> FNLDTEELTAFRVDSAGFGDSVVQYANSWVVVGAPQKITAANQTGGLYQCGYSTGACEPIGLQVPPEAVNMSLGLSLASTTSPSQLLACGPTVHHECGRNMYLTGLCFLLGPTQLTQRLPVSRQECPRQEQDIVFLIDGSGSISSRNFATMMNFVRAVISQFQRPSTQFSLMQFSNKFQTHFTFEEFRRSSNPLSLLASVHQLQGFTYTATAIQNVVH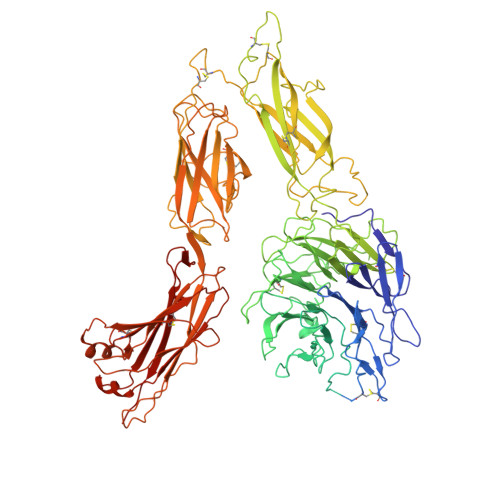RLFHASYGARRDAAKILIVITDGKKEGDSLDYKDVIPMADAAGIIRYAIGVGLAFQNRNSWKELNDIASKPSQEHIFKVEDFDALKDIQNQLKEKIFAIEGTETTSSSSFELEMAQEGFSAVFTPDGPVLGAVGSFTWSGGAFLYPPNMSPTFINMSQENVDMRDSYLGYSTELALWKGVQSLVLGAPRYQHTGKAVIFTQVSRQWRMKAEVTGTQIGSYFGASLCSVDVDSDGSTDLVLIGAPHYYEQTRGGQVSVCPLPRGWRRWWCDAVLYGEQGHPWGRFGAALTVLGDVNGDKLTDVVIGAPGEEENRGAVYLFHGVLGPSISPSHSQRIAGSQLSSRLQYFGQALSGGQDLTQDGLVDLAVGARGQVLLLRTRPVLWVGVSMQFIPAEIPRSAFECREQVVSEQTLVQSNICLYIDKRSKNLLGSRDLQSSVTLDLALDPGRLSPRATFQETKNRSLSRVRVLGLKAHCENFNLLLPSCVEDSVTPITLRLNFTLVGKPLLAFRNLRPMLAADAQRYFTASLPFEKNCGADHICQDNLGISFSFPGLKSLLVGSNLELNAEVMVWNDGEDSYGTTITFSHPAGLSYRYVAEGQKQGQLRSLHLTCDSAPVGSQGTWSTSCRINHLIFRGGAQITFLATFDVSPKAVLGDRLLLTANVSSENNTPRTSKTTFQLELPVKYAVYTVVSSHEQFTKYLNFSESEEKESHVAMHRYQVNNLGQRDLPVSINFWVPVELNQEAVWMDVEVSHPQNPSLRCSSEKIAPPASDFLAHIQKNPVLDCSIAGCLRFRCDVPSFSVQEELDFTLKGNLSFGWVRQILQKKVSVVSVAEITFDTSVYSQLPGQEAFMRAQTTTVLEKYKVHGCGGLENLYFQ>ASTLKSGSKEVENLKKPFMPPREVHVQVTHSMPPQKIEIFKSLDNWAEENILVHLKPVEKCWQPQDFLPDPASDGFDEQVRELRERAKEIPDDYFVVLVGDMITEEALPTYQTMLNTLDGVRDETGASPTSWAIWTRAWTAEENRHGDLLNKYLYLSGRVDMRQIEKTIQYLIGSGMDPRTENSPYLGFIYTSFQERATFISHGNTARQAKEHGDIKLAQICGTIAADEKRHETAYTKIVEKLFEIDPDGTVLAFADMMRKKISMPAHLMYDGRDDNLFDHFSA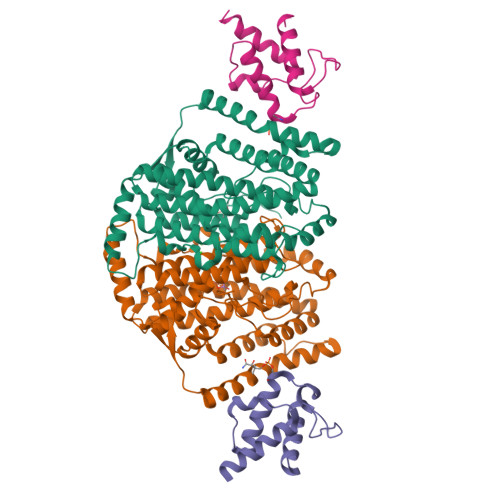VAQRLGVYTAKDYADILEFLVGRWKVDKLTGLSAEGQKAQDYVCRLPPRIRRLEERAQGRAKEAPTMPFSWIFDRQVKL[2x];>AKKETIDKVSDIVKEKLALGADVVVTADSEFSKLGADSLDTVEIVMNLEEEFGINVDEDKAQDISTIQQAADVIEGLLEKKA[2x]>DYKDDDDKLSEHETRLVAKLFKDYSSVVRPVEDHRQVVEVTLGFTLQDIVKADSSTNEVDLVYYEQQRWVDYNLKWNPDDYGGVKKIHIPAADIWTPDITAYSSTRPVQVLSPQIAVVTHDGSVMFIP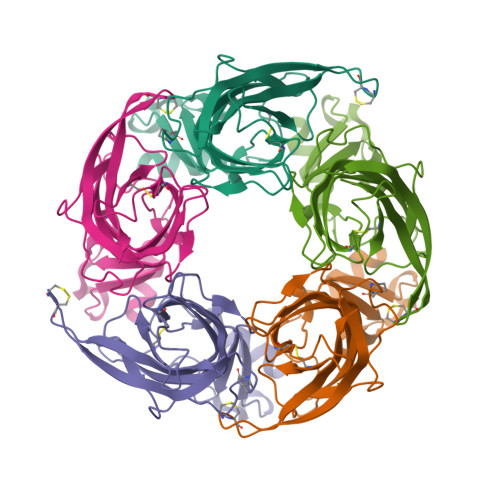AQRLSFMCDPTGVDSEEGATCAVKFGSWVYSGFEIDLKTDTDQVDLSSYYASSKYEILSATQTRQVQHYSCCPEPYIDVNLVVKFRERRAGNGFFRNLFDSR[5x]> MAHHHHHHAAMLRVAVPNKGALSEPATEILAEAGYRRRTDSKDLTVIDPVNNVEFFFLRPKDIAIYVGSGELDFGITGRDLVCDSGAQVRERLALGFGSSSFRYAAPAGRNWTTADLAGMRIATAYPNLVRKDLATKGIEATVIRLDGAVEISVQLGVADAIADVVGSGRTLSQHDLVAFGEPLCDSEAVLIERAGTDGQDQTEARDQLVARVQGVVFGQQYLMLDYDCPRSALKKATAITPGLESPTIAPLADPDWVAIRALVPRRDVNGIMDELAAIGAKAILASDIRFCRF

Many of these FL-regulated enzymes present in pathogenic bacteria, such as the ATP-PRT from Mycobacterium tuberculosis, are essential and have been proposed as attractive targets for antibacterial drug discovery. Because of the common FL fold and functional similarity, the regulatory domain of ATP-PRT has also been associated with the aspartate kinase, chorismate mutase and TyrA (ACT) superfamily. Activation and inhibition of ATP-PRT leads to the same overall conformational tightening of the hexamer. Our data suggest that there is not direct correlation between R- and T-states and active and inactive conformations in ATP-PRT.

In contrast to most screens employed to date, CoSPI identifies molecules that are only active in the presence of a regulator-enzyme complex. This strategy led us to the discovery of 3-(2-Thienyl-l-alanine) (TIH) as a non-essential activator of M. tuberculosis ATP-PRT. As expected on the basis of the overall structural similarity between the two ligands and the results of the competition kinetics experiments, TIH was found to bind in the same allosteric site as l-His, a site defined by opposite and complementing surfaces of two adjacent regulatory FL-like domains. We confirmed the identity of TIH by calculating the anomalous scattering difference map for a data set of the complex collected at 1.8 Å, which exhibited positive density for the sulphur in the thiophenyl moiety and allowed unambiguous assignment of the correct orientation of the ring. Side chains of the residues directly interacting with the ligand assume identical conformations in the two complexes with the only exception of D216. In the ATP-PRT/l-His complex D216 interacts with the l-His side chain via a water molecule-mediated H-bond to ND1, but in the complex with TIH the water molecule is missing and its position occupied by one of two observed conformations for the D216 side chain which is oriented towards the thiophenyl ring. The other noticeable structural difference in the allosteric binding site is the absence in the TIH complex of the H-bond observed between HE2 of l-His and the carbonyl oxygen of A273. The comparison between the structures of both the monomer and the crystallographic hexamer revealed that the l-His inhibited and the TIH activated complexes are highly superimposable and share the same tense (T) conformation so far attributed to the inactive state of the enzyme. The crystallographic structures at 1.8 Å of the ATP-PRT/TIH complex obtained from different crystallization conditions consistently showed the hexamer in a T-state. Addition of either l-His or TIH shifted the equilibrium towards shorter drift times (44.1 and 44.2 ms, respectively), characteristic of the T-state.>MNLPEDAVLVDTRPRPAYEAGHLPGARHLDLSAPKLRLREEAELKALEGGLTELFQTLGLRSPVVLYDEGLTSRLCRTAFFLGLGGLEVQLWTEGWEPYATEKEEPKPERTEVVAKLRRDWLLTADEAARHPLLLDVRSPEEFQGKVHPPCCPRGGRIPGSKNAPLELFL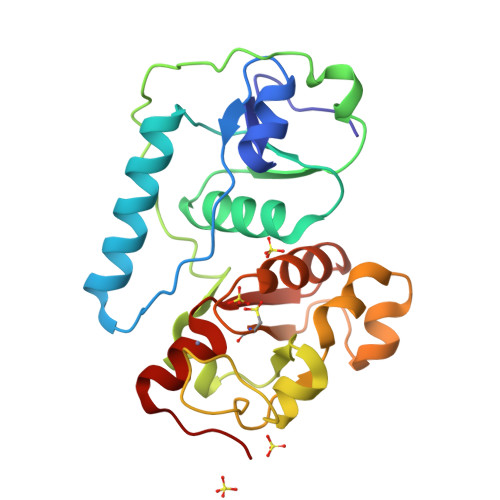SPEGLLERLGLQPGQEVGVYCHSGARSAVAFFVLRSLGVRARNYLGSMHEWLQEGLPTEP[2x]2-{[4-(TRIFLUOROMETHOXY)BENZOYL]AMINO}ETHYL DIHYDROGEN PHOSPHATE | C10 H11 F3 N O6 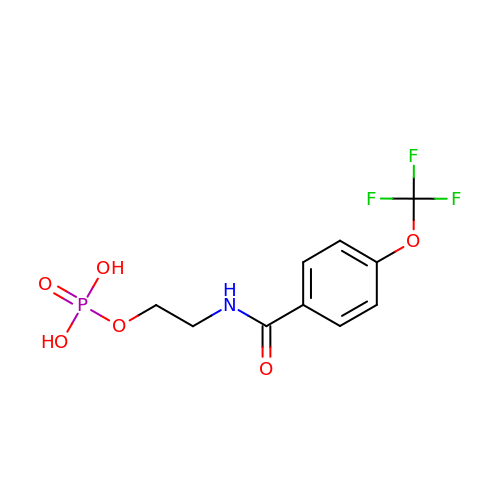P | YAHFSBJEYPSDPU-UHFFFAOYSA-N>MSAIENFDAHTPMMQQYLRLKAQHPEILLFYRMGDFYTLFYDDAKRASQLLDISLTKRGASAGEPIPMAGIPYHAVENYLAKLVNQGESVAICEQIGDPATSKGPVERKVVRIVTPGTISDEALLQERQDNLLAAIWQDSKGFGYATLDISSGRFRLSEPADRETMAAELQRTNPAELLYAEDFAEMSLIEGRRGLRRRPLWEFEIDTARQQLNLQFGTRDLVGFGVENAPRGLCAAGCLLQYAKDTQRTTLPHIRSITMEREQDSIIMDAATRRNLEITQNLAGGAENTLASVLDCTVTPMGSRMLKRWLHMPVRDTRVLLERQQTIGALQDFTAGLQPVLRQVGDLERILARLALRTARPRDLARMRHAFQQLPELRAQLETVDSAPVQALREKMGEFAELRDLLERAIIDTPPVLVRDGGVIASGYNEELDEWRALADGATDYLERLEVRERERTGLDTLKVGFNAVHGYYIQISRGQSHLAPINYMRRQTLKNAERYIIPELKEYEDKVLTSKGKALALEKQLYEELF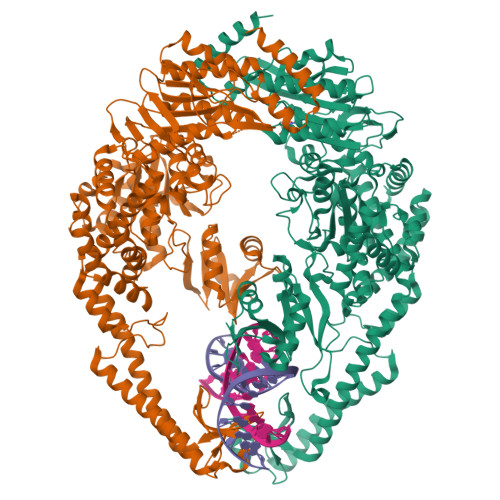DLLLPHLEALQQSASALAELDVLVNLAERAYTLNYTCPTFIDKPGIRITEGRHPVVEQVLNEPFIANPLNLSPQRRMLIITGPNMGGKSTYMRQTALIALMAYIGSYVPAQKVEIGPIDRIFTRVGAADDLASGRSTFMVEMTETANILHNATEYSLVLMDEIGRGTSTYDGLSLAWACAENLANKIKALTLFATHYFELTQLPEKMEGVANVHLDALEHGDTIAFMHSVQDGAASKSYGLAVAALAGVPKEVIKRARQKLRELESIS[2x]> MDYKDDDDKGDHNHRHKHGDPLEVLFQGPGGDPHMSRESNDTIQSDTVRSSSKSDYFRIQLNNQDYYMSKPTFLDPSHGESLPLNQFSQVPNIRVFGALPTGHQVLCHVHGILPYMFIKYDGQITDTSTLRHQRCAQVHKTLEVKIRASFKRKKDDKHDLAGDKLGNLNFVADVSVVKGIPFYGYHVGWNLFYKISLLNPSCLSRISELIRDGKIFGKKFEIYESHIPYLLQWTADFNLFGCSWINVDRCYFRSPVLNSILDIDKLTINDDLQLLLDRFCDFKCNVLSRRDFPRVGNGLIEIDILPQFIKNREKLQHRDIHHDFLEKLGDISDIPVKPYVSSARDMINELTMQREELSLKEYKEPPETKRHVSGHQWQSSGEFEAFYKKAQHKTSTFDGQIPNFENFIDKNQKFSAINTPYEALPQLWPRLPQIEINNNSMQDKKNDDQVNASFTEYEICGVDNENEGVKGSNIKSRSYSWLPESIASPKDSTILLDHQTKYHNTINFSMDCAM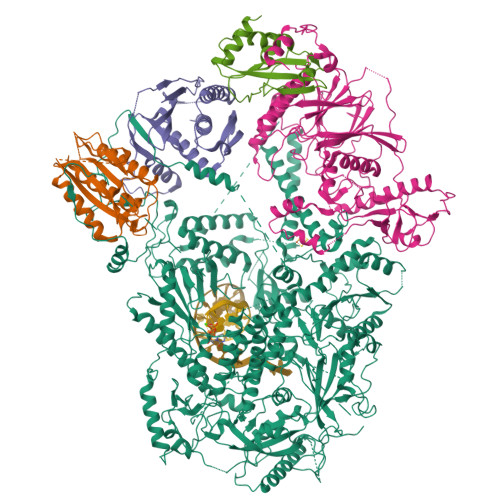TQNMASKRKLRSSVSANKTSLLSRKRKKVMAAGLRYGKRAFVYGEPPFGYQDILNKLEDEGFPKIDYKDPFFSNPVDLENKPYAYAGKRFEISSTHVSTRIPVQFGGETVSVYNKPTFDMFSSWKYALKPPTYDAVQKWYNKVPSMGNKKTESQISMHTPHSKFLYKFASDVSGKQKRKKSSVHDSLTHLTLEIHANTRSDKIPDPAIDEVSMIIWCLEEETFPLDLDIAYEGIMIVHKASEDSTFPTKIQHCINEIPVMFYESEFEMFEALTDLVLLLDPDILSGFEIHNFSWGYIIERCQKIHQFDIVRELARVKCQIKTKLSDTWGYAHSSGIMITGRHMINIWRALRSDVNLTQYTIESAAFNILHKRLPHFSFESLTNMWNAKKSTTELKTVLNYWLSRAQINIQLLRKQDYIARNIEQARLIGIDFHSVYYRGSQFKVESFLIRICKSESFILLSPGKKDVRKQKALECVPLVMEPESAFYKSPLIVLDFQSLYPSIMIGYNYCYSTMIGRVREINLTENNLGVSKFSLPRNILALLKNDVTIAPNGVVYAKTSVRKSTLSKMLTDILDVRVMIKKTMNEIGDDNTTLKRLLNNKQLALKLLANVTYGYTSASFSGRMPCSDLADSIVQTGRETLEKAIDIIEKDETWNAKVVYGDTDSLFVYLPGKTAIEAFSIGHAMAERVTQNNPKPIFLKFEKVYHPSILISKKRYVGFSYESPSQTLPIFDAKGIETVRRDGIPAQQKIIEKCIRLLFQTKDLSKIKKYLQNEFFKIQIGKVSAQDFCFAKEVKLGAYKSEKTAPAGAVVVKRRINEDHRAEPQYKERIPYLVVKGKQGQLLRERCVSPEEFLEGENLELDSEYYINKILIPPLDRLFNLIGINVGNWAQEIVKSKRASTTTTKVENITRVGTSATCCNCGEELTKICSLQLCDDCLEKRSTTTLSFLIKKLKRQKEYQTLKTVCRTCSYRYTSDAGIENDHIASKCNSYDCPVFYSRVKAERYLRDNQSVQREEALISLNDW;>[2x]MNRWVEKWLRVYLKCYINLILFYRNVYPPQSFDYTTYQSFNLPQFVPINRHPALIDYIEELILDVLSKLTHVYRFSICIINKKNDLCIEKYVLDFSELQHVDKDDQIITETEVFDEFRSSLNSLIMHLEKLPKVNDDTITFEAVINAIELELGHKLDRNRRVDSLEEKAEIERDSNWVKCQEDENLPDNNGFQPPKIKLTSLVGSDVGPLIIHQFSEKLISGDDKILNGVYSQYEEGESIFGSLF;> GPGGDLHMDALLTKFNEDRSLQDENLSQPRTRVRIVDDNLYNKSNPFQLCYKKRDYGSQYYHIYQYRLKTFRERVLKECDKRWDAGFTLNGQLVLKKDKVLDIQGNQPCWCVGSIYCEMKYKPNVLDEVINDTYGAPDLTKSYTDKEGGSDEIMLEDESGRVLLVGDFIRSTPFITGVVVGILGMEAEAGTFQVLDICYPTPLPQNPFPAPIATCPTRGKIALVSGLNLNNTSPDRLLRLEILREFLMGRINNKIDDISLIGRLLICGNSVDFDIKSVNKDELMISLTEFSKFLHNILPSISVDIMPGTNDPSDKSLPQQPFHKSLFDKSLESYFNGSNKEILNLVTNPYEFSYNGVDVLAVSGKNINDICKYVIPSNDNGESENKVEEGESNDFKDDIEHRLDLMECTMKWQNIAPTAPDTLWCYPYTDKDPFVLDKWPHVYIVANQPYFGTRVVEIGGKNIKIISVPEFSSTGMIILLDLETLEAETVKIDI;> MDQKASYFINEKLFTEVKPVLFTDLIHHLKIGPSMAKKLMFDYYKQTTNAKYNCVVICCYKDQTIKIIHDLSNIPQQDSIIDCFIYAFNPMDSFIPYYDIIDQKDCLTIKNSYELKVSESSKIIERTKTLEEKSKPLVRPTARSKTTPEETTGRKSKSKDMGLRSTALLAKMKKDRDDKETSRQNELRKRKEENLQKINKQNPEREAQMKELNNLFVEDDLDTEEVNGGSKPNSPKETDSNDKDKNNDDLEDLLETTAEDSLMDVPKIQQTKPSETEHSKEPKSEEEPSSFIDEDGYIVTKRPATSTPPRKPSPVVKRALSSSKKQETPSSNKRLKKQGTLESFFKRKAK>GIDPFTKHGQKECDNALRQLETVRELLENPVQPINDMSYFGCLDSVMENSKVLGEAMTGISQNAKNGNLPEFGDAIATASKALCGFTEAAAQAAYLVGVSDPNSQAGQQGLVEPTQFARANQAIQMACQSLGEPGCTQAQVLSAATIVAKHTSALCNSCRLASARTANPTAKRQFVQSAKEVANSTANLVKTIKALDGDFTEENRAQCRAATAPLLEAVDNLSAFASNPEFSSVPAQISPEGRAAMEPIVISAKTMLESAGGLIQTARALAVNPRDPPRWSVLAG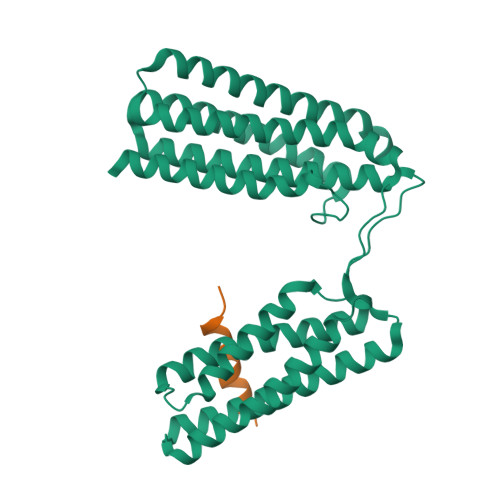HSRTVSDSIKKLITSMRDKAPGQL[2x];>DSEIDQLFRIFRALGTP[2x]> DTVGRPLPHLAAAMQASGEAVYCDDIPRYENELFLRLVTSTRAHAKIKSIDVSEAQKVPGFVCFLSADDIPGSNETGLFNDETVFAKDTVTCVGHIIGAVVADTPEHAERAAHVVKVTYEDLPAIITIEDAIKNNSFYGSELKIEKGDLKKGFSEADNVVSGELYIGGQDHFYLETHCTIAIPKGEEGEMELFVSTQNAMKTQSFVAKMLGVPVNRILVRVKRMGGGFGGKET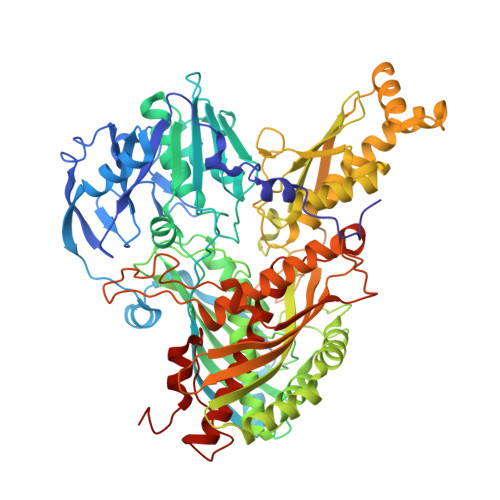RSTLVSVAVALAAYKTGHPVRCMLDRNEDMLITGGRHPFLARYKVGFMKTGTIVALEVDHYSNAGNSRDLSHSIMERALFHMDNCYKIPNIRGTGRLCKTNLSSNTAFRGFGGPQALFIAENWMSEVAVTCGLPAEEVRWKNMYKEGDLTHFNQRLEGFSVPRCWDECLKSSQYYARKSEVDKFNKENCWKKRGLCIIPTKFGISFTVPFLNQAGALIHVYTDGSVLVSHGGTEMGQGLHTKMVQVASKALKIPISKIYISETSTNTVPNSSPTAASVSTDIYGQAVYEACQTILKRLEPFKKKNPDGSWEDWVMAAYQDRVSLSTTGFYRTPNLGYSFETNSGNAFHYFTYGVACSEVEIDCLTGDHKNLRTDIVMDVGSSLNPAIDIGQVEGAFVQGLGLFTLEELHYSPEGSLHTRGPSTYKIPAFGSIPTEFRVSLLRDCPNKKAIYASKAVGEPPLFLGASVFFAIKDAIRAARAQHTNNNTKELFRLDSPATPEKIRNACVDKFTT> MGSSHHHHHHSSGENLYFQGHMSAADTAEDLPEQFRIRRDKRARLLAQGRDPYPVAVPRTHTLAEVRAAHPDLPIDTATEDIVGVAGRVIFARNSGKLCFATLQDGDGTQLQVMISLDKVGQAALDAWKADVDLGDIVYVHGAVISSRRGELSVLADCWRIAAKSLRPLPVAHKEMSEESRVRQRYVDLIVRPE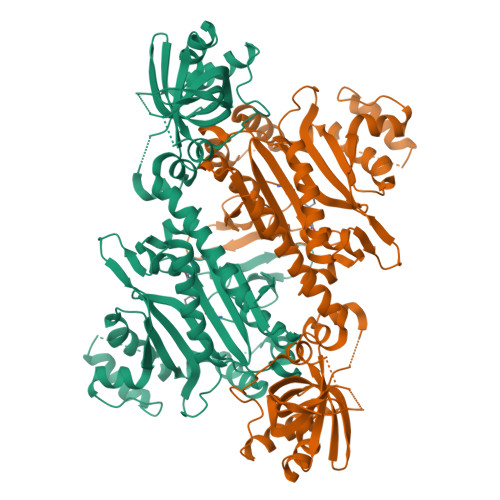ARAVARLRIAVVRAIRTALQRRGFLEVETPVLQTLAGGAAARPFATHSNALDIDLYLRIAPELFLKRCIVGGFDKVFELNRVFRNEGADSTHSPEFSMLETYQTYGTYDDSAVVTRELIQEVADEAIGTRQLPLPDGSVYDIDGEWATIQMYPSLSVALGEEITPQTTVDRLRGIADSLGLEKDPAIHDNRGFGHGKLIEELWERTVGKSLSAPTFVKDFPVQTTPLTRQHRSIPGVTEKWDLYLRGIELATGYSELSDPVVQRERFADQARAAAAGDDEAMVLDEDFLAALEYGMPPCTGTGMGIDRLLMSLTGLSIRETVLFPIVRPHSN>MATEFGTAVNHADLVERLVQFLTASPDLVAAGQAYEKVFDNTIPASGTAIAVRQVTLRAPGLGGTDAIYMGIQSYGDTALDYYNLRLMGGTAFNPGAIPPGGDYWTAFANYSPRVQLLAWNQPMPYWFFANGRRFWIVVKVSTIYESAGAGFILPPCPPSQYPYPLAVVGSYRGDVATRWSDVSDRHRGISSPYERSCYLRDPAGRWLGFTVDGGAANESDYNNRTLLPLGCGRYAGSSDTVVKQLRDS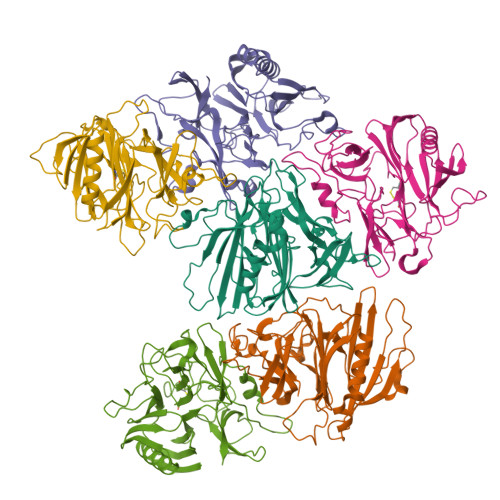FGKFPLKALQFVTRETEGRRYLGDFDGAFYVPTLNSGAEDVIVEDGVDHVVFQTAWRSGNPWLYAIRKD[3x];>MAYFTGTANNPADLLAKVRVHAESLGWVTDRASASEWLCHNADGYWSFNAGANQFQMAGNTGFDNSLAWNAQPGNSVQNNPYSSKGPTVAQLSGGPFTRYHLFATAAYLHLHVEIAAGQFRPVMIGSLNKRGVGYTGGQYVCGSFIYTPGQALTNNWSSHPFDGYHIQYSNSSCMLRLDGLDGGPSPEWLPFDYTTNVPRRVVGPGRGNYSSQYHPDVGLIDASANELNSSTTTVPCAIYAFGAQQRSRYVGEVPDFGICNMAFLAPGDPLVVGSDTWRVYPLLQRGTATDFDSTSAWVGYCFRVVE[3x]> SSLGSQKERLLDELTLEGVARYMQSERCRRVICLVGAGISTSAGIPDFRSPSTGLYDNLEKYHLPYPEAIFEISYFKKHPEPFFALAKELYPGQFKPTICHYFMRLLKDKGLLLRCYTQNIDTLERIAGLEQEDLVEAHGTFYTSHCVSASCRHEYPLSWMKEKIFSEVTPKCENCQSLVKPDIVFFGESLPARFFSCMQSDFLKVDLLLVMGTSLQVQPFASLISKAPLSTPRLLINKEKAGQSDPFLGMIMGLGGGMDFDS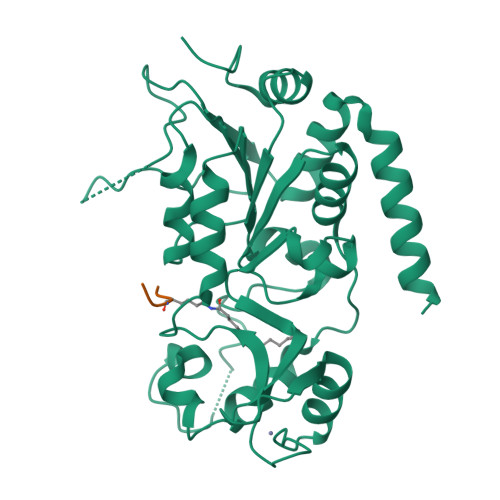KKAYRDVAWLGECDQGCLALAELLGWKKELEDLVRREHASIDAQ;> PRKQL AMINO-AUSTRALINE | C8 H16 N2 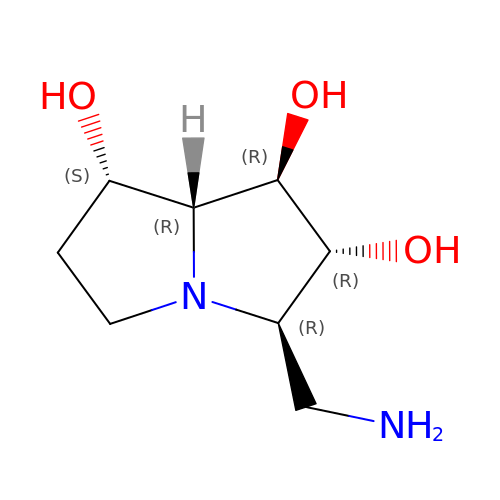O3 | RTYGUSZVNGAYPW-OZRXBMAMSA-N> MGSSHHHHHHSSGLVPAGSHMAGTKKGVSAAAFSGVTAALGDVGARWFYTWAAD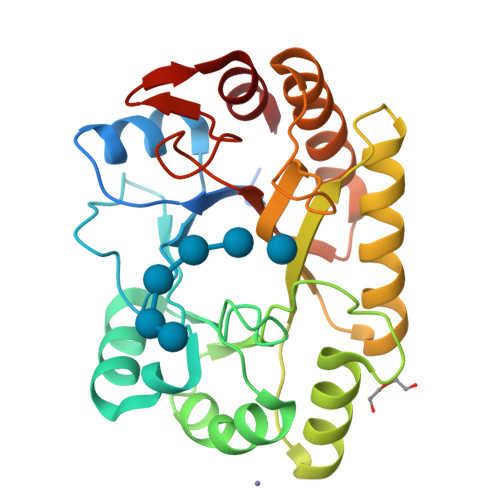PQGITAPAGTEFVPMIWGRDSVTADQLQRAKAAGSTLLAFNEPDLAGQANMSVETALDLWPQLQATGMRLGAPAVAYGGDTPGGWLDRFMSGAAARGYRVDFIPLHWYGGDFSAAATGQLQSYLQAVYNRYHRPIWLTAYALTDFSGSTPRYPSAAEQADFVSRSTAMLNGLSFVERYAWFSLSTSTTPTGLYTGTTPNSSGVAYRAAG4-{[1-(2-{[({5-[(3-carboxypropanoyl)amino]-2,4-dimethoxyphenyl}sulfonyl)amino]methyl}phenyl)piperidin-4-yl]methoxy}-4-oxobutanoic 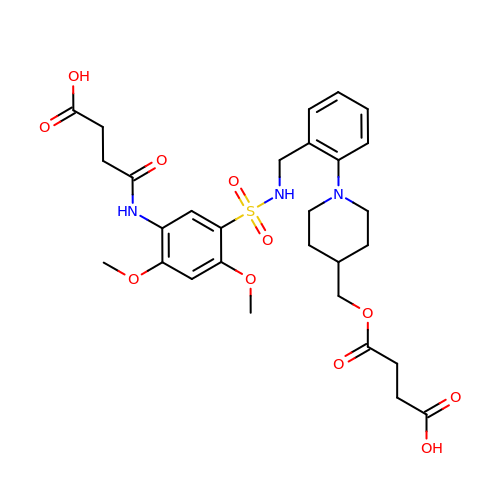acid | C29 H37 N3 O11 S | PRDHHOYRFMTLDT-UHFFFAOYSA-N> MNHKVHMQYDIVAVTASAHDGNLPENTIDGNLSTRWSANGSGQYITFDLGSAKTVNQVKAAWYNGDSRTSGFSISLGSDPASLTEVYSGTSSGQTNALESYS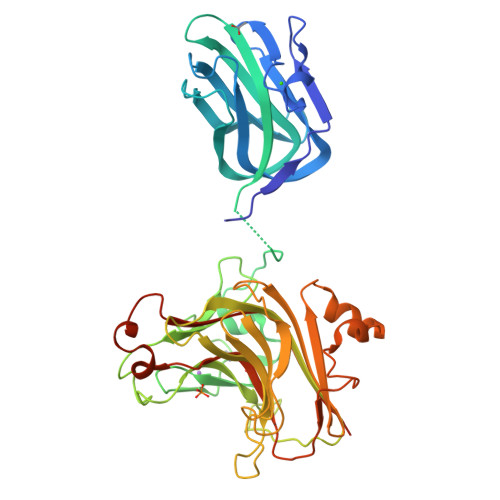FTATTARYIRITGFGNSSNTWNSITEVAIFHAGEEGDGNEEAPGTAQIPSDLMSNCNQWKITYPDGSEDKTLCGEANNEYWFVNEDKNAMVFRAPIRSNNGTTPNSSYVRSELRERKEDGSADIYWTTTGTHVVYVKQAITQLPIVKDHLVATQIHGDKSAGIDDAMVMRLEGNHLFASFNGGKLRSDLTIKTNYNLGTVHEVIFEVINGKHYLYYSEDGKLAEAYANGSAAAYLIKDGGNDYVMDLNYDQSYFKIGNYTQSNSEKEGSYTGDPNNYGEVVVYDYFVSHQHHHHHH>[3x]MSIEKLKAALPEYA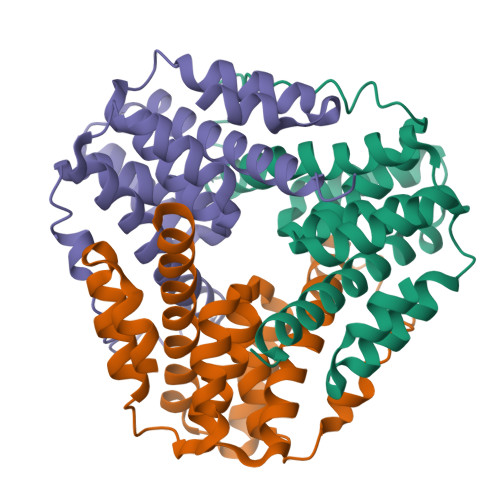KDIKLNLSSITRSSVLDQEQLWGTLLASAAATRNPQVLADIGAEATDHLSAAARHAALGAAAIMGMNNVFYRGRGFLEGRYDDLRPGLRMNIIANPGIPKANFELWSFAVSAINGCSHCLVAFEHTLRTVGVDREAIFEALKAAAIVSGVAQALATIEALSPS> MTVFRQENVDDYYDTGEELGSGKFAVVKKCREKSTGLQYAAKFIKKRRTKSSRRGVSREDIEREVSILKEIQHPNVITLHEVYENKTDVIL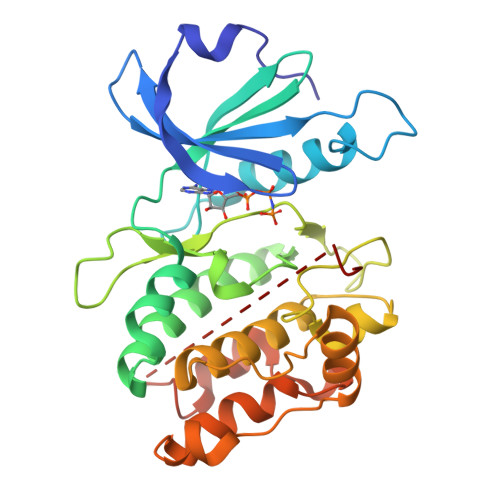ILELVAGGELFDFLAEKESLTEEEATEFLKQILNGVYYLHSLQIAHFDLKPENIMLLDRNVPKPRIKIIDFGLAHKIDFGNEFKNIFGTPEFVAPEIVNYEPLGLEADMWSIGVITYILLSGASPFLGDTKQETLANVSAVNYEFEDEYFSNTSALAKDFIRRLLVKDPKKRMTIQDSLQHPWIKPKDTQQALSSAWSHPQFEK>MKELIRKLTEAFGPSGREEEVRSIILEELEGHIDGHRIDGLGNLIVWKGSGEKKVILDAHIDEIGVVVTNVDDKGFLTIEPVGGVSPYMLLGKRIRFENGTIGVVGMEGETTEERQENVRKLSFDKLFIDIGANSREEAQKMCPIGSFGVYDSGFVEVSGKYVSKAMDDRIGCAVIVEVFKRIKPAVTLYGVFSVQEEVGLVGASVAGYGVPADEAIAIDV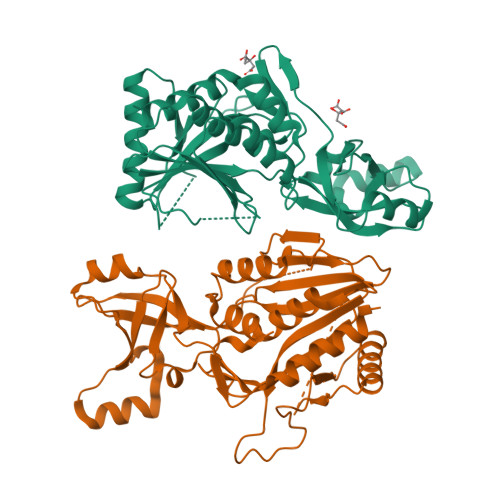TDSADTPKAIKRHAMRLSGGPALKVKDRASISSKRILENLIEIAEKFDIKYQMEVLTFGGTNAMGYQRTREGIPSATVSIPTRYVHSPSEMIAPDDVEATVDLLIRYLGA[2x]>MQNSVIIVDKNGRLVYLVENPGGSVANSKAATVTGKLVHANFG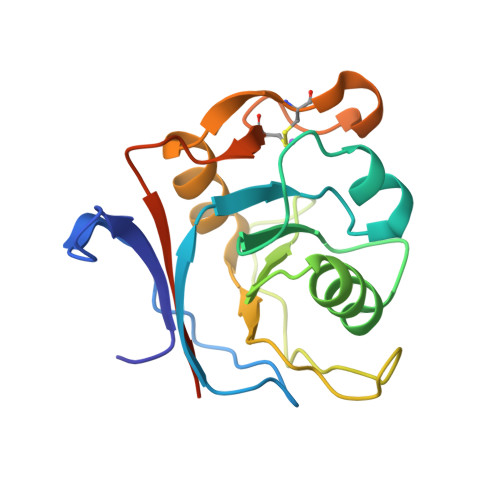TKKDFEDLYTPVNGSIVIVRAGKITFAEKVANAESLNAIGVLIYMDQTKFPIVNAELSFTGKGKSGIPVQTISRAAAEKLFGNMEGDCPSDWKTDSTCRMVTSESKNVKLTVSGSGSLEHHHHHH[2x]> SEAEARPTNFIRQIIDEDLASGKHTTVHTRFPPEPNGYLHIGHAKSICLNFGIAQDYKGQCNLRFDDTNPVKEDIEYVESIKNDVEWLGFHWSGNVRYSSDYFDQLHAYAIELINKGLAYVDELTPEQIREYRGTLTQPGKNSPYRDRSVEENLALFEKMRAGGFEEGKACLRAKIDMASPFIVMRDPVLYRIKFAEHHQTGNKWCIYPMYDFTHCISDALEGITHSLCTLEFQDNRRLYDWVLDNITIPVHPRQYEFSRLNLEYTVMSKRKLNLLVTDKHVEGWDDPRMPTISGLRRRGYTAASIREFCKRIGVTKQDNTIEMASLESCIREDLNENAPRAMAVIDPVKLVIENYQGEGEMVTMPNHPNKPEMGSRQVPFSGEIWIDRADFREEANKQYKRLVLGKEVRLRNAYVIKA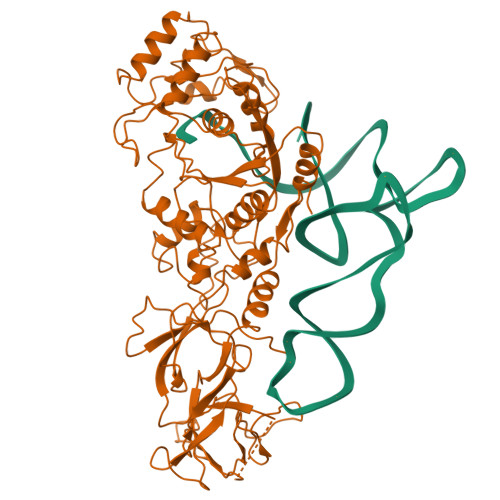ERVEKDAEGNITTIFCTYDADTLSKDPADGRKVKGVIHWVSAAHALPVEIRLYDRLFSVPNPGAADDFLSVINPESLVIKQGFAEPSLKDAVAGKAFQFEREGYFCLDSRHSTAEKPVFNRTVGLRDTWAKVGE>[4x]MSVGTFSLPALPYAYDALEPSISAQIVELHHSKHHQTYVTNLNNALKTYSTALAANDVPSQIALQAAIKFNGGGHINHSLFWENLCPASSPDADPASAPELTAEIAKTWGSLDKFKEAMGK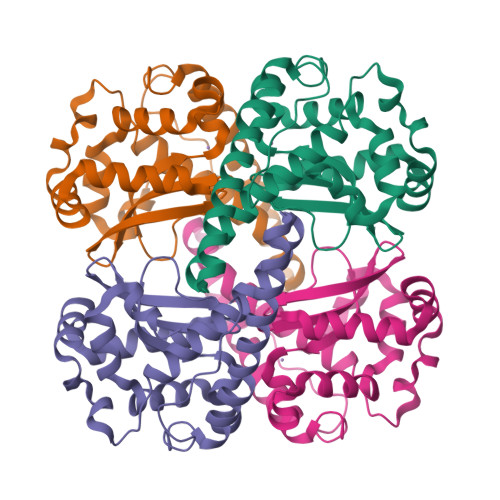ALLGIQGSGWGWLVKEGSGLRIVTTKDQDPVVGGEVPVFGIDMWEHAYYLQYLNGKAAYVDNIWKVINWKTAEQRFKGDREDAFKILKASL> GSPPIINHFHFSKDIKEGERQQVICGLKSGDPPFTFSWLKDGIDIKNFPEINIVDVPVSYISVLVISSVEAKHIGNYTCIIKNSNGMDSYTATLMMKVPPRWVKEPTDVAATLGSRLTIDCSATGYPQPQITWDKLTDRSEHQLPVGSDSQRTLASNGSLTFLRVDESDKGVYICQAYNGIGNGLQKKIHLTVHVAPKVKEDFTVITVRKGFTAHLKCEVFGEPPLNIIWKKEDKIIAGEKGSRFETLQENTANGATSDTLINDSQQNDSGIYTCHVSSQFGEAEGKIQLVVLES

Recently, a shortened Dscam (sDscam) gene family with tandemly arrayed 5′ cassettes in Chelicerata species has been identified, which encodes ∼50–100 isoforms. Chelicerata sDscams could be classified into two subfamilies, sDscamα and sDscamβ, containing one and two variable Ig domains, respectively. Crystal structures and cell aggregation assays demonstrated that both α and β subfamilies of sDscam used Ig1 for the isoform-specific trans recognition in a hand-in-hand manner. Furthermore, the cis interactions were established by the three FNIII domains of sDscam, which assemble into a cross fold with a kink between FNIII2 and FNIII3.

We also determined the crystal structures of sDscam Ig1 from another chelicerate species Limulus polyphemus (isoforms α7 and β3v7) to provide insights into the conservation of sDscam trans recognition within Chelicerata. These crystal structures of Ig fragments were determined at 1.3–3.1 Å resolutions. The crystal structures of sDscam Ig1 from both M. martensii and L. polyphemus revealed a common assembly of antiparallel homodimer for both α and β subfamilies of sDscam. Similarly, sDscam Ig1 also employs the ABED face to form an antiparallel homodimer. The trans interactions of Chelicerata sDscam were mediated exclusively through the Ig1 domain for both sDscamα and sDscamβ subfamilies. For both α and β subfamilies, wild type sDscams lead to cell aggregation, while truncation of Ig1 domain, but not other Ig domains, completely abolished cell aggregation. This finding supported the functional significance of Ig1 in mediating the trans recognition of sDscam, which was consistent with our structural analysis.>GSHMKISEFLHLALPEEQWLPTISGVLRQFAEEECYVYERPPCWYLGKGCQARLHINADGTQATFIDDAGEQKWAVDSIADCARRFMAHPQVKGRRVYGQVGFNFAAHARGIAFNAGEWPLLTLTVPREELIFEKGNVTVYADSADGCRRLCEWVKEASTTTQ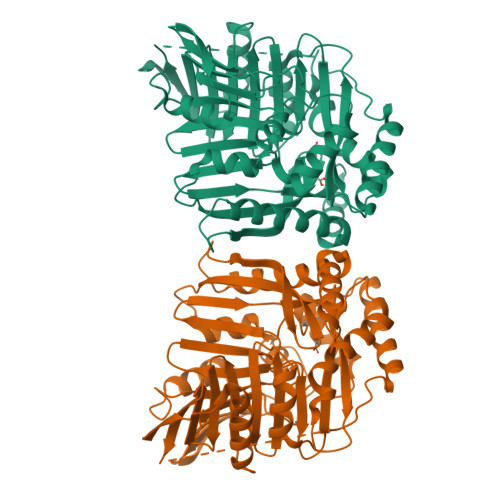NAPLAVDTALNGEAYKQQVARAVAEIRRGEYVKVIVSRAIPLPSRIDMPATLLYGRQANTPVRSFMFRQEGREALGFSPELVMSVTGNKVVTEPLAGTRDRMGNPEHNKAKEAELLHDSKEVLEHILSVKEAIAELEAVCLPGSVVVEDLMSVRQRGSVQHLGSGVSGQLAENKDAWDAFTVLFPSITASGIPKNAALNAIMQIEKTPRELYSGAILLLDDTRFDAALVLRSVFQDSQRCWIQAGAGIIAQSTPERELTETREKLASIAPYLMV[2x]> MALYPIKSLGAVGVIADQAPTDLAPNAFTNAINARFVEQRVFKTGGNAPLSYVDEDKDLTPLSFVSMPFDYYSAGNSFLVVGTNKKLYKLTDESLTDISRKVATVTKKASASIKIYPVVSQIVPKESTISMNFNQTKNLEVSLLPADANNTNLIWEVSNSSYGSITVDPSDSKLATLTSFEKEGNLVVTISTANESVVAQIAVNIIDGDSGIFLSQDTVTIRKGGTTTLTAVTGKTPVTWSSNNASIVSVTPNANSLTAVITANGEGNVTITADNGTKTASCEIVSIPQIDSISLSQSDVTVSRGSQYILTATLSPANAPNQNITWTSSNPNIATVSGTSTQGTINALLAGFTEITATTEEGNRVAVCTVRVDLAGRTMRTSAMAFAAPVSESVETQEEEVVTPPESEETVYFAEPTSGIDTSGMYEGNNFYDYSNVNDIEGFARASLLATPLSSVTLDIVSASLDVGEEIVITATASPEGEYSYQWSVDKTGYVSTTSVTGKSIKLVALRKGEINVTCTVSQMTQKDYDAFDDYPWYHAVISNCAVATTHYETPQVKEFESEYFVDLPGWGEQTVVDNDGNPSVKKFNWKCERVRSFNNRLFALNMREANASGVTTNYPLRLRWSNFANENKAPTLWDDFAYDRVVSSDLASNIVGQTQALENGYAGYIDLADSNGSLIDILPLKDYLFVYTEFETYIGSPTNNTYQPLMFKKLFNDSGILAPECVVEVEGSHFVVTQNDVILHNGATKKSIASNRVKNMLINEVCLVNPLATRVHLHQDKKEVWVLYVGPGEPKESFACTKAAVWN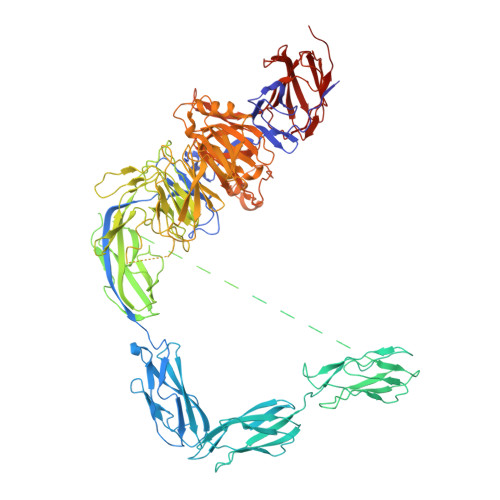YEFDTWSFRTIPYAQCIGLVDPPVLERGPIWSDFQEITWDDPSIKELVWRKDATNFRQRVTIVGSFLKGFYQVDVGALDYFYDRLNDVVIEKPLEMRLERTGIDFDNVTNEWNQKHINRFRPQTTGSGTYIFEAGGSQFSNEYGHPHTSKTYTIGVDRHVSVRLNHPYLFYNVIDNDVNSNAAINGLTIEFAVGGRR> MAHHHHHHVDDDDKMCSSNNLSKSNTSNSSKTSSSSKKITLTFWNLFTGEPAKTKVKEIIDQWNKENPNVQIVESVTENDAYKTKIKAAIAANEAPDIFQTWAGGFSQPFVEAGKVLQLDSYLNDGTKDQLLPGSFDNVTYNGKIYGIPFDQQASVLYINKELFDKYNVKVPTTFSELIDAIKTFKSKGVTP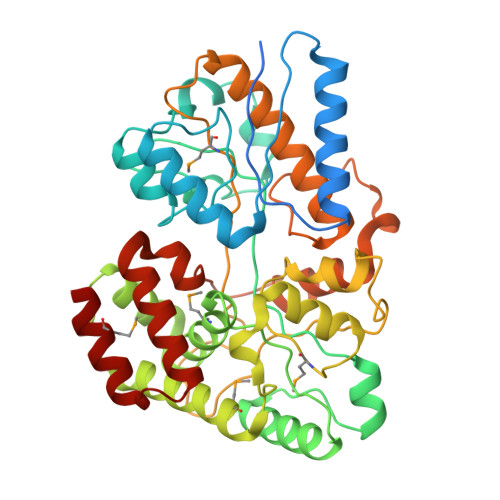FALGEKDEWPGMWYYDMIALREGGVQLTRDALNGKASFDNQAFTDAAQKLQDMVNAGAFDSGFMGLTRDEATAEFNQGKAAMYFGGNFDAAAFVSDPSSLVKGKIEAVRFPTIEGGKGDPTEYIGGTVGALMVSANSKYKDEAVRAAKYLAKQLSDMDYLIATGLPAWKYDNIDQSKVDPLEIQIMNNIVANAKGSVPAWDIYLSGDAAQTHKDLVAQLFAKQITPEEYSKQMQQKINGK> MFRLGTTPRATTY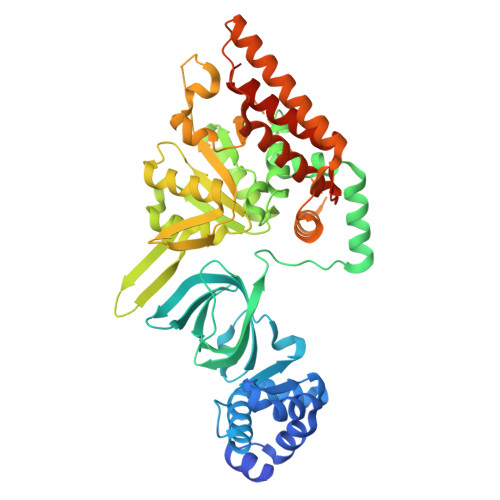DPDARIGEVASRFGLPTRVLIEIVRTESFQRSLARVTSGKPVVLDLRELDSDLASWIATHARLVEPALRELVRTVAPDVEPRVRFRGLPHRFRRVERIRPMDGALISIEGVVREVRGAERLEHAIVDTGSELVAVRLHGHRLGPGLRVEILGIVRSATLDALEVHKKDPIPEVHPDPAELEEFRELADKDPLTTFARAIAPLPGAEEVGKMLALQLFSCVGKNSERLHVLLAGYPVVCSEILHHVLDHLAPRGVYVDLRRTELTDLTAVLKEDRGWALRAGAAVLADGGILAVDHLEGAPEPHRWALMEAMDKGTVTVDGIALNARCAVLAAINPGEQWPSDPPIARIDLDQDFLSHFDLIAFLGVDPRPGEPEEQDTEVPSYTLLRRYLLYAIREHPAPELTEEARKRLEHWYETRREEVEERLGMGLPTLPVTRRQLESVERLAKAHARMRLSDDVEPEDVDIAAELVDWYLETAMQIPGGDEIRISSLKP2-O-phosphono-beta-D-glucopyranose 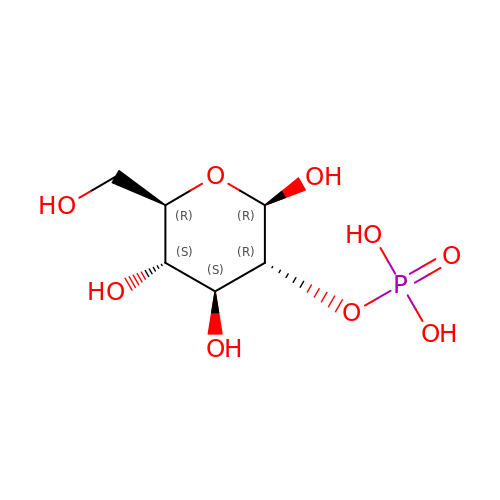| C6 H13 O9 P | SIUIENVKPUKAHD-VFUOTHLCSA-N> MRNELEEMQRRADQLADESLESTRRMLQLVEESKDAGIRTLVMLDEQGEQLDRVEEGMN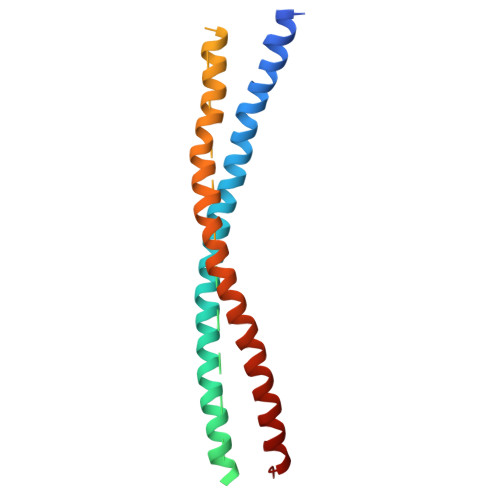HINQDMKEAEKNLKDLGKFCGLCVCPCNKLKSSDAYKKAWGNNQDGVVASQPARVVDEREQMAISGGFIRRVTNDARENEMDENLEQVSGIIGNLRHMALDMGNEIDTQNRQIDRIMEKADSNKTRIDEANQRATKMLG4-[[(1S,3R)-5-oxidanyl-2-adamantyl]amino]-1H-pyrrolo[2,3-b]pyridine-5-carboxamide | C18 H22 N4 O2 | 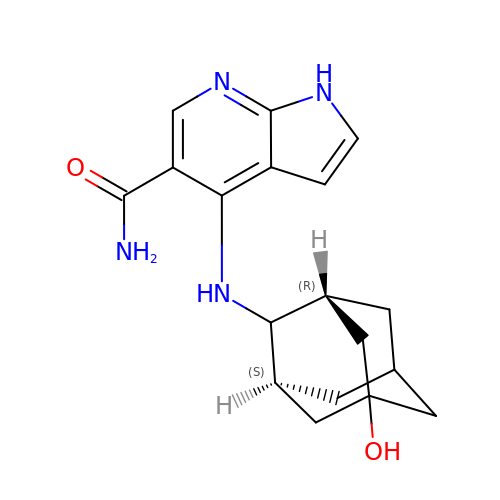DREIJXJRTLTGJC-ZKVNVPQCSA-N Decarboxylated Myriocin | 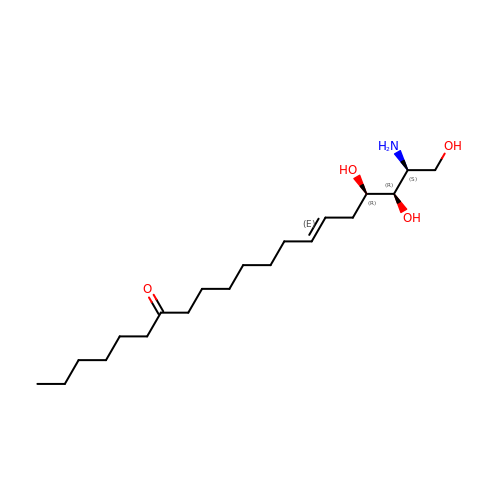C20 H39 N O4 | NXVWIVNGDXWOCH-INRCJLNUSA-N We have discovered orally active small molecules that inhibit TNF activity both in vitro and in vivo. The compounds bind to a pocket in the centre of the TNF trimer formed by the movement of the TNF monomers, stabilising the distorted trimer, which leads to reduced signalling through TNFR1. Analytical size exclusion suggests that the asymmetric trimer only binds to two receptors, consistent with the structural data showing significant distortion at one receptor binding interface. We show here an approach to inhibiting TNF through allosteric binding using small, drug-like, orally available molecules that we believe stabilise a naturally occurring conformer of TNF.

After screening for compound-dependent crystallisation conditions, crystals diffracting to 2.5 Å were obtained for UCB-6876. The structure shows three TNF monomers in the asymmetric unit (ASU) and clear electron density for one molecule of UCB-6876 bound at the centre of the TNF trimer. The compound was buried within the space between the three TNF monomers and did not make any contact with solvent. The key interactions appeared to be the hydrogen bond from a benzimidazole N atom to Y151C (Y151 in chain C) and π stacking of the benzimidazole with Y59C. The 2,5-dimethylbenzyl moiety of UCB-6876 filled a hydrophobic pocket, assigned as Site 2, with compound TNF interactions composed of Y59A, Y119B and L57B. The asymmetry of the compound-bound TNF trimer results in minor distortion at two of the receptor-binding sites and a more significant change at the AC binding site (i.e., the receptor-binding site formed at the interface of the arbitrarily assigned A and C monomers in the crystal lattice). There is a clear opening of the AC site because of monomer A twisting and tilting down and away from monomer C. That UCB-6876 binds to a low abundance form of TNF is consistent with the slow on-rate observed by SPR, since the association rate constant is dependent on binding site access and concentration. As indicated by the crystal structure, once bound it is completely buried between the TNF monomers, explaining the slow dissociation rate.

>VRSSSRTPSDKPVAHVVANPQAEGQLQWLNRRANALLANGVELRDNQLVVPSEGLYLIYSQVLFKGQGCPSTHVLLTHTISRIAVSYQTKVNLLSAIKSPCQRETPEGAEAKPWYEPIYLGGVFQLEKGDRLSAEINRPDYLDFAESGQVYFGIIAL[3x]>[2x]MGSHHHHHHDITSLYKKAGSAAAVLEENLYFGGSFTMANVNKTPGKTRRAEVAGGGFA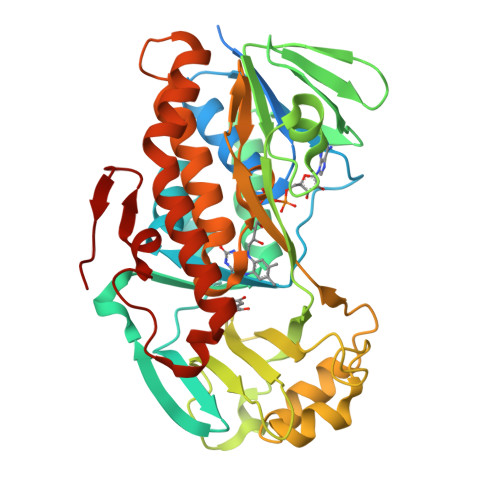GLTAAIALKQNGWDVRLHEKSSELRAFGAGIYLWHNGLRVLEGLGALDDVLQGSHTPPTYETWMHNKSVSKETFNGLPWRIMTRSHLHDALVNRARALGVDISVNSEAVAADPVGRLTLQTGEVLEADLIVGADGVGSKVRDSIGFKQDRWVSKDGLIRLIVPRMKKELGHGEWDNTIDMWNFWPRVQRILYSPCNENELYLGLMAPAADPRGSSVPIDLEVWVEMFPFLEPCLIEAAKLKTARYDKYETTKLDSWTRGKVALVGDAAHAMCPALAQGAGCAMVNAFSLSQDLEEGSSVEDALVAWETRIRPITDRCQALSGDYAANRSLSKGNMFTPAALEAARYDPLRRVYSWPQ> GPLGSMGKKSRVKTQKSGTGATATVSPKEILNLTSELLQKCSSPAPGPGKEWEEYVQIRTLVEKIRKKQKGLSVTFDGKREDYFPDLMKWASENGASVEGFEMVNFKEEGFGLRATRDIKAEELFLWVPRKLLMTVESAKNSVLGPLYSQDRILQAMGNIALAFHLLCERASPNSFWQPYIQTL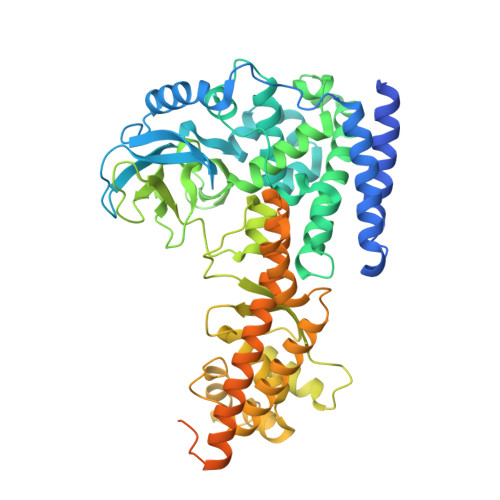PSEYDTPLYFEEDEVRYLQSTQAIHDVFSQYKNTARQYAYFYKVIQTHPHANKLPLKDSFTYEDYRWAVSSVMTRQNQIPTEDGSRVTLALIPLWDMCNHTNGLITTGYNLEDDRCECVALQDFRAGEQIYIFYGTRSNAEFVIHSGFFFDNNSHDRVKIKLGVSKSDRLYAMKAEVLARAGIPTSSVFALHFTEPPISAQLLAFLRVFCMTEEELKEHLLGDSAIDRIFTLGNSEFPVSWDNEVKLWTFLEDRASLLLKTYKTTIEEDKSVLKNHDLSVRAKMAIKLRLGEKEILEKAVKSAAVNREYYRQQMEEKAPLPKYEESNLGLLESSVGDSRLPLVLRNLEEEAGVQDALNIREAISKAKATENGLVNGENSIPNGTRSENESLNQESKRAVEDAKGSSSDSTAGVKE>[2x]MHHHHHHENLYFQSNAMASLKRFQTLVPLDHKQGTLFEIIGEPKLPKWFHVECLEDPKRLYVEPRLLEIMFGKDGEHIPHLESMLHTLIHVNVWGPERRAEIWIFGPPPFRR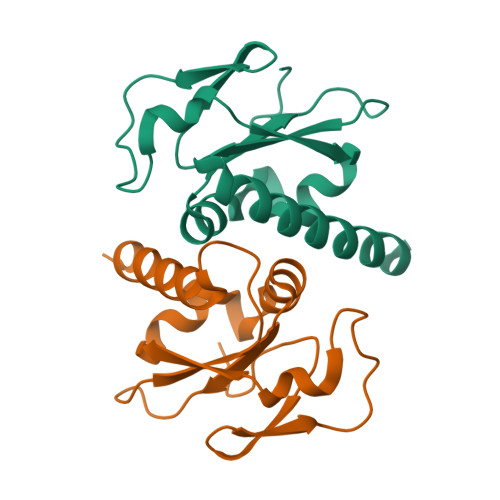DVDRMLTDLAHYCRMKLMEIEALEAGVE>MADKELKFLVVDDFSTMRRIVRNLLKELGFNNVEEAEDGVDALNKLQAGGYGFVISDWNMPNMDGLELLKTIRADGAMSALPVLMV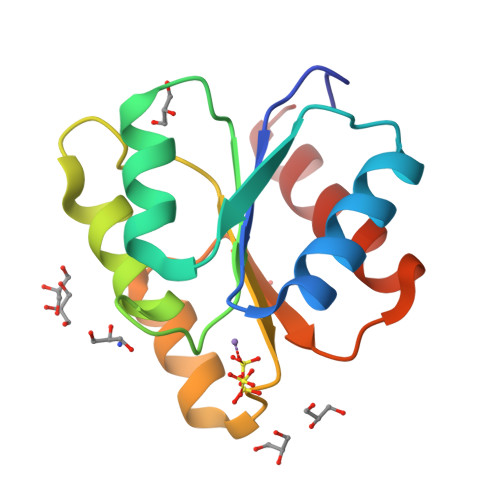TAEAKKENIIAAAQAGASGYVVKPFTPATLEEKLNKIFEKLGM[2x]> MKITSSNFATIATSENFAKLSV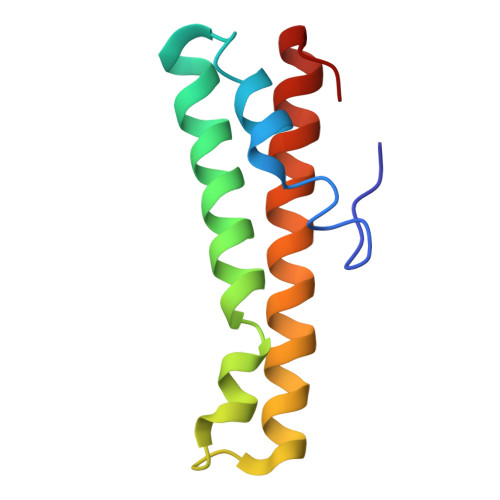LPKNHREPIKGLFKSAVEQFSSARDFFKNENYSKELAEKFNKEAVNEAVEKLQKAIDLAEKQGIQF> GIEDLITEVAQGALTLSLPKQQDSLPDTKASGPAHSKEVPALTAVETGATNPLVPSDTVQTRHVIQRRSRSESTIESFFARGACVAIIEVDNEEPTTRAQKLFAMWRITYKDTVQLRRKLEFFTYSRFDMELTFVVTANFTNTNNGHALNQVYQIMYIPPGAPTPKSWDDYTWQTSSNPSIFYTYGAAPARISVPYVGLANAYSHFYDGFAKVPLKTDANDQIGDSLYSAMTVDDFGVLAIRVVNDHNPTKVTSKVRIYMKPKHVRVWCPRPPRAVPYYGPGVDYKDNLNPLSEKGLTTY;> SPNVEACGYSDRVLQLTIGNSTITTQEAANSVVAYGRWPEFIRDDEANPVDQPTEPDVATCRFYTLDTVMWGKESKGWWWKLPDALRDMGLFGQNMYYHYLGRSGYTVHVQCNASKFHQGALGVFAIPEYCLAGDSDKQRYTSYANANPGEKGGKFYSQFNRDTAVTSPKREFCPVDYLLGCGVLLGNAFVYPHQIINLRTNNSATIVLPYVNAMAIDSMVKHNNWGIAILPLSPLDFAQESSVEIPITVTIAPMCSEFNGLRNVTAPKFQ;> GLPVLNTPGSNQYLTSDNYQSPCAIPEFDVTPPIDIPGEVKNMMELAEIDTMIPLNLENTKRNTMDMYRVTLSDSADLSQPILCFSLSPASDPRLSHTMLGEVLNYYTHWAGSLKFTFLFCGSMMATGKILVAYAPPGAQPPTSRKEAMLGTHVIWDLGLQSSCTMVVPWISNVTYRQTTQDSFTEGGYISMFYQTRIVVPLSTPKSMSMLGFVSACNDFSVRLLRDTTHISQSALPQ;> MGAQVSSQKVGAHENSNRAYGGSTINYTTINYYKDSASNAASKQDYSQDPSKFTEPLKDVLIKTAPALN

Poliovirus (PV), a member of the Picornaviridae, is the causative agent of poliomyelitis and destroys motor neurons in the central nervous system causing paralysis or even death. Genome-free (empty) PV particles, such as recombinantly expressed VLPs, do not undergo the final maturation cleavage of VP0 into VP2 and VP4, which rearranges the proteins on the inside of the virus capsid with a concomitant increase in particle stability. Therefore, to produce an effective vaccine from empty particles, it will be necessary to stabilize the particles to maintain the desired antigenic phenotype. To confirm the authenticity of the plant-expressed PV VLPs, we have determined structures of the stabilized plant-expressed PV3 SktSC8 sVLPs by cryo-EM in the absence and presence of the GPP3 pocket-binding compound.

The structure of the PV3 SktSC8 sVLP was solved to 3.6 Å resolution by cryo-EM and showed that the particle is very similar to that of wt PV3 Sabin strain, demonstrating that recombinant plant-expression of PV VLPs can produce authentic particles with the correct antigenic features. The overall architecture of the plant-expressed PV3 SktSC8 sVLP preserves all the structural features characteristic of native conformation particles including the canyon depression around the fivefold vertex of the capsid. The only significant changes are on the interior of the particle, where the N-terminal region of the uncleaved VP0 in the empty sVLPs is less well ordered than the corresponding regions of VP4 and VP2 in the mature virus (residues corresponding to VP2 1–11 and VP4 1–25 and 41–69 are not visible in the sVLPs). In addition, the N-terminus of VP1 from residues 1 to 65 is disordered in the sVLP structures; such disordering is commonly seen in empty particles although these are usually in the expanded C antigenic form. Although the pocket is “open” as expected for a structure with D antigenicity, very little density is observed for a pocket factor molecule in the VP1 protein for the PV3 SktSC8 sVLP structure at 3.6 Å resolution, although one or more pocket factors may be present at very low occupancy. However, it is likely that some VP1 pockets are occupied since the pocket has not collapsed (structure is native antigenicity) and some weak density is observed. It is likely that the VP1 pocket is partly occupied with a heterogeneous mixture of pocket factors, acquired from the plant cell expression system. The mutations are distributed evenly across the protomer, and are involved in either stabilizing the hydrophobic core of individual protomer subunits (VP1 T105N and VP3 L85F), increasing the hydrophobic packing between protomers within the pentamer of the VLP (VP2 L215M and VP3 H19Y), or, in one case (VP1 F132L), modulating the lining of the VP1 pocket where the pocket factor binds.>HHHHHHDMLNSLHAITGKFKTQSRLVVGLGDESVYETSIRLLRNYGVPYIPGSAIKGVTRHLTYYVLAEFINEGNDFYKRAKTVQDAFMKGDPKEILSNAKVPERCSRLCKEFLRIFGEKKVPEIIDELIRIFGTQKKEGEVVFFDAIPIAEEIADKPILELDIMNPHYGPYYQSGEKNVPPPGDWYDPIPIFFLTVPKDVPFLVAVGGRDRELTEKAFSLVKLALRDLGVGAKTS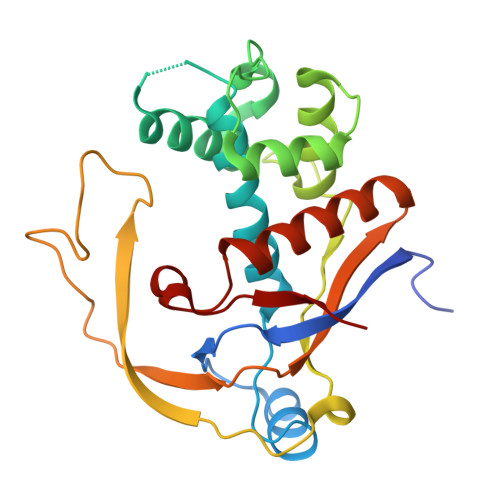LGYGRLVEYV[2x]>[2x]SRPI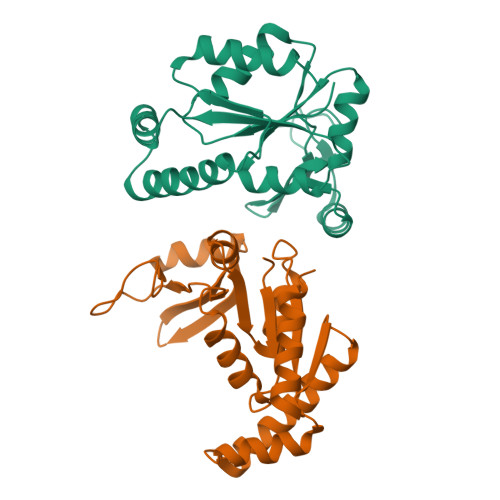VISGPSGTGKSTLLKKLFAEYPDSFGFSVSSTTRTPRAGEVNGKDYNFVSVDEFKSMIKNNEFIEWAQFSGNYYGSTVASVKQVSKSGKTCILDIDMQGVKSVKAIPELNARFLFIAPPSVEDLKKRLEGRGTETEESINKRLSAAQAELAYAETGAHDKVIVNDDLDKAYKELKDFIFAEK6-O-phosphono-alpha-D-mannopyranose | C6 H13 O9 P | 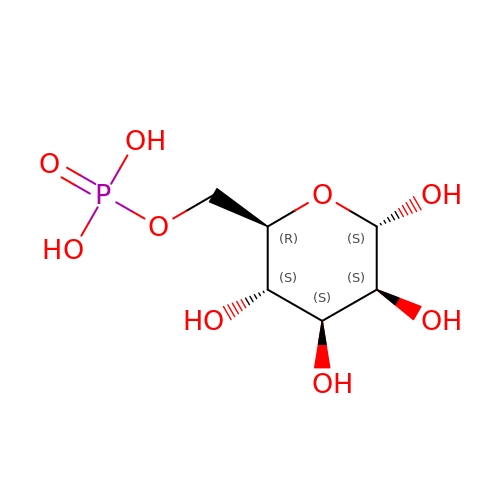NBSCHQHZLSJFNQ-PQMKYFCFSA-N>[2x]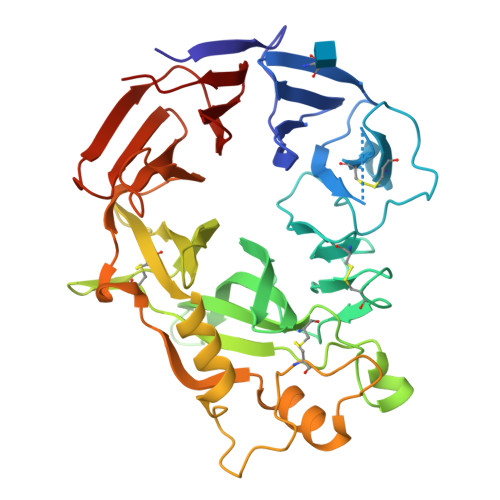SIEWHKFETSEEIISTYLLDDVLYTGVNGAVYTFSNNKLNKTGLTNNNYITTSIKVEDADKDTLVCGTNNGNPKCWKIDGSDDPKHRGRGYAPYQNSKVTIISYNECVLSDINISKEGIKRWRRFDGPCGYDLYTADNVIPKDGLRGAFVDKDGTYDKVYILFTDTIGSKRIVKIPYIAQMCLNDEGGPSSLSSHRWSTFLKVELECDIDGRSYRQIIHSRTIKTDNDTILYVFFDSPYSKSALCTYSMNTIKQSFSTSKLEGYTKQLPSPAPGICLPAGKVVSHTTFEVIEKYNVLDDIIKPLSNQPIFEGPSGVKWFDIKEKENEHREYRIYFIKENSIYSFDTKSKQTRSSQVDARLFSVMVTSKPLFIADIGIGVGMPQ>[2x]GSQIHVDTMKVINDPIHGHIELHPLLVRIINTPQFQRLRYIKQLGGGYYVFPGASHNRFEHSLGVGYLAGCLVHALGEKQPELQISERDVLCVQIAGLCHDLGHGPFSHMFDGRFIPLARPEVKWTHEQGSVMMFEHLINSNGIKPVMEQYGLIPEEDICFIKEQIVGPLESPVEDSLWPYKGRPENKSFLYEIVSNKRNGIDVDKWDYFARDCHHLGIQNNFDYKRFIKFARVCEVDNELRICARDKEVGNLYDMFHTRNSLHRRAYQHKVGNIIDTMITDAFLKADDYIEITGAGGKKYRISTAIDDMEAYTKLTDNIFLEILYSTDPKLKDAREILKQIEYRNLFKYVGETQPTGQIKIKREDYESLPKEVASAKPKVLLDVKLKAEDFIVDVINMDYGMQEKNPIDHVSFYCKTAPNRAIRITKNQVSQLLPEKFAEQLIRVYCKKVDRKSLYAARQYFVQWCADRNFTKPQDGDVIAPLITPQKKEWNDSTSVQNPTRLREASKSRVQLFKDDPM

Sterile alpha motif and HD domain-containing protein 1 (SAMHD1) is an important regulator of cellular 2′-deoxynucleoside-5′-triphosphate (dNTP) in mammalian cells. Although the HD-domain contains the active site, dNTP hydrolysis requires assembly of SAMHD1 into homo-tetramers. Here, sequences at the N and C termini of the HD-domain stabilise inter-monomer protein–protein interactions and incorporate four pairs of allosteric nucleotide-binding sites, AL1 and AL2, which regulate the enzyme through combined binding of G-based (AL1) and 2′-deoxynucleoside (AL2) triphosphates. Using combined biophysical and X-ray structural studies incorporating nucleotide analogues along with mutagenesis experiments we have now discovered that SAMHD1 uses a bi-metallic Fe–Mg centre to catalyse dNTP hydrolysis in a reaction similar to those catalysed by HD domains in both human and bacterial phosphodiesterase PDE enzymes.

Co-crystal structures were determined using either wild-type (wt) wt-SAMHD1(109-626) or a D137N-SAMHD1(109-626) AL1 allosteric site mutant that generally produced higher resolution diffraction than wt co-crystals. A further effect of the D137N substitution is that D137N-SAMHD1 is activated by xanthosine-5′-triphosphate (XTP) rather than GTP through AL1-binding but nevertheless maintains comparable catalytic parameters for dNTP hydrolysis as those observed for wt-SAMHD1 and GTP. We first determined structures of two co-complexes of D137N-SAMHD1(109-626) in the presence of Mg2+, which is required for tetramer assembly and catalysis, with (i) XTP (AL1) and dAMPNPP (AL2 and active site), and (ii) XTP (AL1) and dGMPNPP (AL2 and active site). However, with regards to the active-site nucleotide configuration and metal ion content, it is apparent there are significant differences that are crucial for understanding the catalytic mechanism of SAMHD1. This is most evident in our highest resolution structure, D137N-SAMHD1(109-626)-XTP-dAMPNPP-Mg, that clearly demonstrates how three octahedrally coordinated metal ions Fe, Mg2 and Mg3, support catalysis through interactions with the bound substrate, as detailed below. Inspection of the D137N-XTP-dAMPNPP structure reveals the key residues that position the α-phosphate proximal to the HD motif-coordinated iron, and are likely important for dNTP hydrolysis. In particular, the nucleotide 5′ oxygen, as well as non-bridging α-phosphate oxygens of dAMPNPP make hydrogen bonds with SAMHD1 side chains Arg164, His210 and His215, whereas the β- and γ-phosphates are coordinated by Mg2. The two non-bridging α-phosphate oxygens form coordinate bonds with Fe and Mg3, one phosphate oxygen coordinates Fe with an Fe–O bond distance of 2.2 Å and the second phosphate oxygen coordinates Mg3, with an Mg–O bond distance of 2.3 Å.> MSTAEFAQLLENSILSPDQNIRLTSETQLKKLSNDNFLQFAGLSSQVLIDENTKLEGRILAALTLKNELVSKDSVKTQQFAQRWITQVSPEAKNQIKTNALTALVSIEPRIANAAAQLIAAIADIELPHGAWPELMKIMVDNTGAEQPENVKRASLLALGYMCESADPQSQALVSSSNNILIAIVQGAQSTETSKAVRLAALNALADSLIFIKNNMEREGERNYLMQVVCEATQAEDIEVQAAAFGCLCKIMSLYYTFMKPYMEQALYALTIATMKSPNDKVASMTVEFWSTICEEEIDIAYELAQFPQSPLQSYNFALSSIKDVVPNLLNLLTRQNEDPEDDDWNVSMSAGACLQLFAQNCGNHILEPVLEFVEQNITADNWRNREAAVMAFGSIMDGPDKVQRTYYVHQALPSILNLMNDQSLQVKETTAWCIGRIADSVAESIDPQQHLPGVVQACLIGLQDHPKVATNCSWTIINLVEQLAEATPSPIYNFYPALVDGLIGAANRIDNEFNARASAFSALTTMVEYATDTVAETSASISTFVMDKLGQTMSVDENQLTLEDAQSLQELQSNILTVLAAVIRKSPSSVEPVADMLMGLFFRLLEKKDSAFIEDDVFYAISALAASLGKGFEKYLETFSPYLLKALNQVDSPVSITAVGFIADISNSLEEDFRRYSDAMMNVLAQMISNPNARRELKPAVLSVFGDIASNIGADFIPYLNDIMALCVAAQNTKPENGTLEALDYQIKVLEAVLDAYVGIVAGLHDKPEALFPYVGTIFQFIAQVAEDPQLYSEDATSRAAVGLIGDIAAMFPDGSIKQFYGQDWV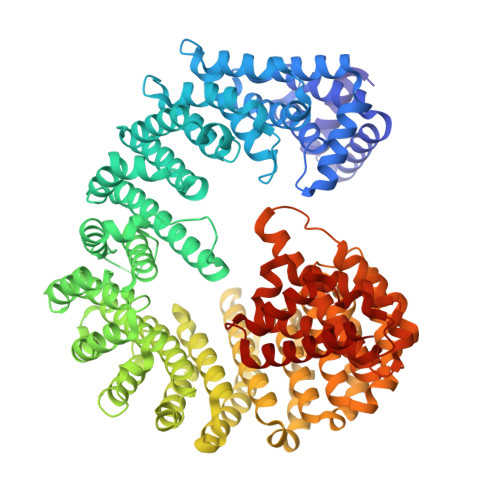IDYIKRTRSGQLFSQATKDTARWAREQQKRQLSL> MAQANFGVVGMAVMGKNLALNVESRGYTVAIYNRTTSKTEEVFKEHQDKNLVFTKTLEEFVGSLEKPRRIMLMVQAGAATDATIKSLLPLLDIGDILIDGGNTHFPDTMRRNAELADSGINFIGTGVSGGEKGALLGPSMMPGGQKEAYDLVAPIFEQIAAKAPQDGKPCVAYMGANGAGHYVKMVHNGIEYGDMQLIAESYDLLKRILGLSNAEIQ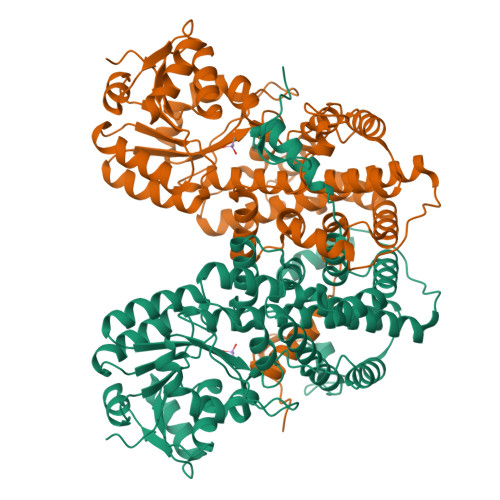AIFEEWNEGELDSYLIEITKEVLKRKDDEGEGYIVDKILDKAGNKGTGKWTSESALDLGVPLPLITESVFARYISTYKDERVKASKVLSGPALDFSGDKKEVIEKIRKALYFSKIMSYAQGFAQLRKASEEFDWDLPYGTIAQIWRAGCIIRAEFLQNITDAFDKDSELENLLLDDYFVDITKRYQEAVRDVVSLAVQAGTPIPTFTSAISYYDSYRSENLPANLIQAQRDYFGAHTYERTDKAGIFHYDWYTED>[2x]MASREEIFSKVKSIISEK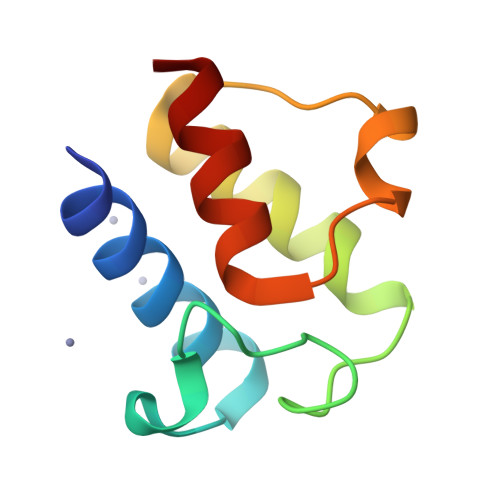LGVDESQVTEEAKLIDDLGADSLDLVDLVMDFESEFGVKVDDADLEKISTVGDIVSYIEKKLG> IVGGKVCPKGECPWQVLLLVNGAQLCGGTLINTIWVVSAAHCFDKIKNWRNLIAVLGEHDLSEHDGDEQSRRVAQVIIPSTYVPGTTNHDIALLR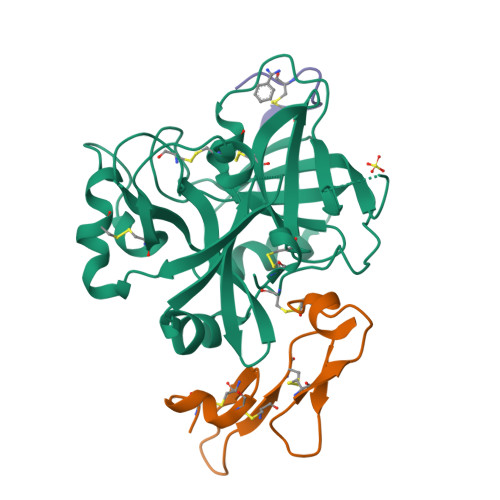LHQPVVLTDHVVPLCLPERTFSERTLAFVRFSLVSGWGQLLDRGATALELMVLNVPRLMTQDCLQQSRKVGDSPNITEYMFCAGYSDGSKDSCKGDSGGPHATHYRGTWYLTGIVSWGQGCATVGHFGVYTRVSQYIEWLQKLMRSEPRPGVLLRAPFP;> ICVNENGGCEQYCSDHTGTKRSCRCHEGYSLLADGVSCTPTVEYPCGKIPILEKRNASKPQGR;> EEWEVLCWTWETCER> MHHHHHHHAVRASEISRVYEAYPEKKATLYFLVLGFLALIVGSLFGPFQALNYGNVDAYPLLKRLLPFVQSYYQGLTLHGVLNAIVFTQLFAQAIMVYLPARELNMRPNMGLMWLSWWMAFIGLVVFALPLLANEATVLYTFYPPLKGHWAFYLGASVFVLSTWVSIYIVLDLWRRWKAANPGKVTPLVTYMAVVFWLMWFLASLGLVLEAVLFLLPWSFGLVEGVDPLVARTLFWWTGHPIV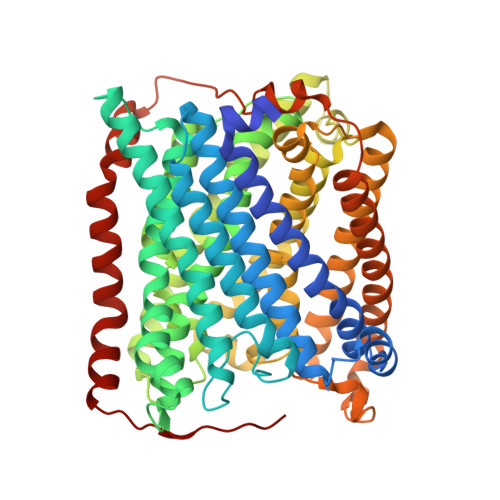YFWLLPAYAIIYTILPKQAGGKLVSDPMARLAFLLFLLLSTPVGFHHQFADPGIDPTWKMIHSVLTLFVAVPSLMTAFTVAASLEFAGRLRGGRGLFGWIRALPWDNPAFVAPVLGLLGFIPGGAGGIVNASFTLDYVVHNTAWVPGHFHLQVASLVTLTAMGSLYWLLPNLTGKPISDAQRRLGLAVVWLWFLGMMIMAVGLHWAGLLNVPRRAYIAQVPDAYPHAAVPMVFNVLAGIVLLVALLLFIYGLFSVLLSRERKPELAEAPLPFAEVISGPEDRRLVLAMDRIGFWFAVAAILVVLAYGPTLVQLFGHLNPVPGWRLW> MATTAKQAEAVEDSDINPWTGQRHSERYFKILKARRKLPVNKQRQEFLDLYHNNQILVFVGETGSGKTTQIPQYVLYDELPHQTGKLIACTQPRRVAAMSVAQRVADELDVKLGEEVGYSIRFENKTSSKTLLKYMTDGQLLREAMHDRDMSRYSCIILDEAHERTLATDILMALLKQLSERRKDLKIIVMSATLDAQKFQSYFFNAPLLAVPGRTHPVEIFYTPEAERDYVEAAIRTVLQIHACEPEGDILLFLTGEEEIEDACRRISLEVDEMIRESDAGPMSVYPLYGTLPPHQQQRIFEKAPQPFRPGGRPGRKCIVATNIAETSLTIDGIVYVVDPGFSKQKIYNPRTRVESLLVSPISKASAQQRAGRAGRTRPGKCFRLYTEEAFKKELIEQTYPEILRSNLSNTVLELKKLGVEDLVHFDLMDPPAPETMMRALEELNYLACLDDDGELTPLGNLASEFPLDPALAVMLISSPEFYCSNEILSITSLLSVPQIWVRPANARKRADEMKAQFAHPDGDHLTLLNAYHAYKGAEARGEDMKKWCHEHFLSYRHLSSADNVRAQLKKIMETHGIELVSTPFHDKNYYTNIRRALLAGFFMQVAMRESSNSKVYKTVKDEQLVLIHPSTTVTTPYEWVVYNEFVLTTKQYVRTVTNIRPEWLLEIAPVYYDLSTFQKGEIKNALTRVAEKIRRQQAMKASKAWSHPQFEK

In the course of this process, Prp43 acts at the latest stage of the splicing cycle and it is required to dismantle the intron-lariat spliceosome into the excised lariat and the U2•U5•U6 snRNPs. Prp43 action is also essential for ribosome biogenesis. For these crystallization approaches, an N-terminally truncated version of Prp43 from C. thermophilum was used (ctPrp43ΔN), which lacks the first 60 amino acids.

Crystals of ctPrp43ΔN•ADP•BeF3- in the presence of the U16-RNA were obtained in the space group P6122 and diffracted up to 2.62 Å. In addition to the ADP•BeF3- and a central magnesium ion at the active site, seven out of the 16 nucleotides of the RNA as well as one additional phosphate group were traceable in the electron density (for an omit map of the RNA see Figure 1—figure supplement 1a). Hence, this complex is referred to here as ctPrp43ΔN•U7•ADP•BeF3-. By this ctPrp43ΔN•U7•ADP•BeF3- complex structure, insights into the sequence-unspecific RNA-binding mechanism of a genuine DEAH-box helicase were obtained. ctPrp43 consists of six different domains: an N-terminal extension (residues 1–96), the RecA1 (97–273) and RecA2 (274–458) domains, and the C-terminal domains which were assigned as degenerate winged helix domain (459–526), ratchet-like domain (527–640) and oligosaccharide binding-fold domain (641–764). The RecA-like domains and the C-terminal domains appear to be stably associated by multiple interactions and form a tunnel inside the Prp43 molecule which is the binding site of the U7-RNA. The 5’ end of the RNA is located at the RecA2 domain and the 3’ RNA end is situated at the RecA1 domain. For the first three nucleotides at the 5’ end (U1–U3) two alternative conformations are observed. Most of these interactions are formed between the sugar-phosphate backbone of the RNA and the RecA1, RecA2 or the ratchet-like domain. On the contrary, the uracil moieties do not interact with the helicase with the exception of a hydrogen bond of U3 with the Ser 555 main-chain carboxyl group from the ratchet-like domain and a base stack between the U1 and Arg 562 which only occurs in one of the two alternative conformations. Prp43 was known to bind RNA in a sequence-independent manner which is explained by the ctPrp43ΔN•U7•ADP•BeF3- complex structure revealing the almost entire absence of interactions between the bases of the RNA and Prp43.> MEGLEAYDYHLPPEQIAQEGVEPRDMARLMVVYREGPFRVAHKRVRDLPEFLRPGDVLVFNESKVIPARLLARKPTGGKVEILLVRERSPGLWEALLGPARKAPPGTRLLLLSPKDLAPVPGL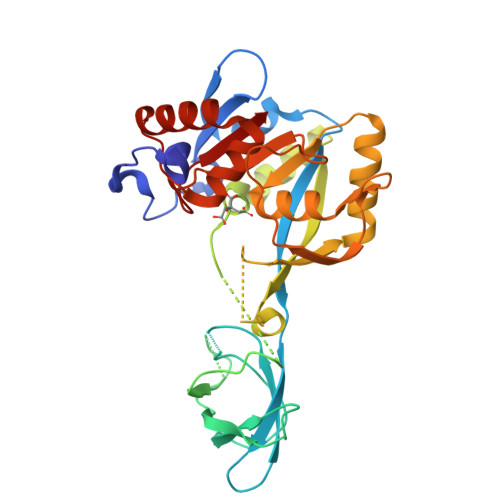QAEVVAVEEDGVRLLRFQGDLVAHLEEVGEVPLPPYIKAKIPMERYQTVYARRPGSVAAPTAGLHFTPELLERLREMGVELRFLTLHVGPGTFRPVKGDPEKHEMHAEPYAIPEEVAEAVNRAKAEGRRVVAVGTTVVRALESAYREGVGVVAGEGETRLFIRPPYTFKVVDALFTNFHLPRSTLLMLVAAFLGRERTLEAYRLAVAEGYRFYSLGDAMLIL>MKHHHHHHPMVKEYKTITQIAGPLIFVEKTEPVGYNEIVNIKMGDGTVRRGQVLDSSADIVVVQVFEGTGGLDKDCGVIFTGETLKLPASVDLLGRILSGSGEPRDGGPRIVPDQLLDINGAAMNPYARLPPKDFIQTGISTIDGTNTLVRGQKLPIFSASGLPHNEIALQIARQASVPGSESAFAVVFAAMGITNEEAQYFMSDFEKTGALERAVVFLNLADDPAVERIVTPRMALTAAEYLAYEHGMHVLVILTDITNYAEALRQMGAARNEVPGRRGYPGYMYTDLATLYERAGIVKGAKGSVTQIPILSMPGDDITHPIPDLSGYITEGQIVVA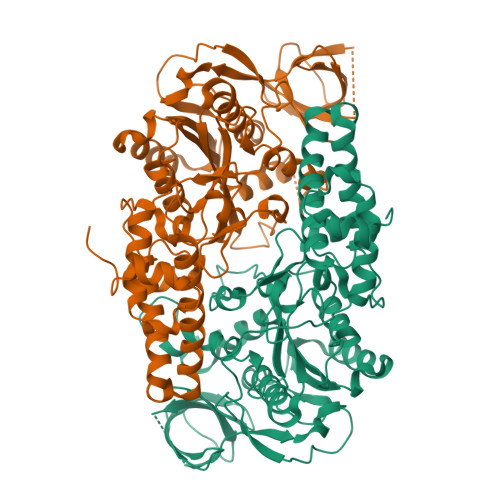RELHRKGIYPPINVLPSLSRLMNSGIGAGKTREDHKAVSDQMYAGYAEGRDLRGLVAIVGKEALSERDTKFLEFADLFEDKFVRQGRNENRTIEDTLEIGWQILTHLPENQLGRIDNKYIQKYHPAHRKAK[2x]> G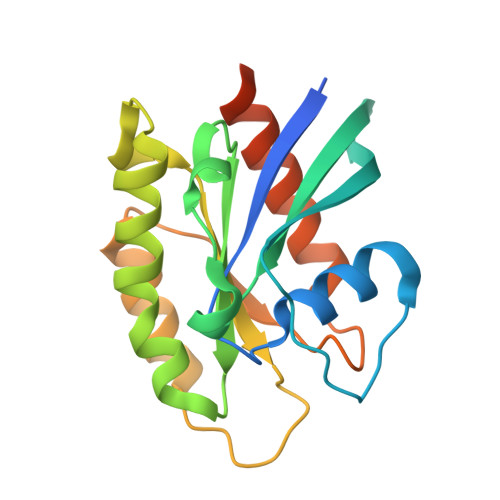SAMGSTSRKKVLLKVIILGDSGVGKTSLMNQYVNKKFSNQYKATIGADFLTKEVMVDDRLVTMQIWDTAGLERFQSGVAFYRGADCCVLVFDVTAPNTFKTLDSWRDEFLIQASPRDPENFPFVVLGNKIDLENRQVATKRAQAWCYSKNNIPYFETSAKEAINVEQAFQTIARNALKQETEVELYNEFPEPIKLDKN One such target is the enzyme O-acetyltransferase A (OatA). This extracellular enzyme modifies the essential bacterial cell wall component peptidoglycan and thereby makes it resistant to the lytic action of lysozyme, our first line of defense against invading pathogens. It uses a catalytic triad of Ser-His-Asp to transfer acetyl groups specifically to the C-6 hydroxyl group of muramoyl residues within peptidoglycan. The overall structure of SpOatAC adopts an atypical α/β hydrolase fold, where the core parallel β-sheet contains five strands (β1 - β5) sandwiched between seven α-helices (α1–α7) forming a shallow and solvent exposed putative active site pocket.

Unequivocal identification of Ser438 in SpOatAC as the catalytic nucleophile was made using the mechanism-based, irreversible inhibitor of Ser esterases methanesulfonyl fluoride (MSF). SpOatAC treated with this reagent lacked detectable catalytic activity and X-ray crystallographic analysis of a native crystal soaked with MSF revealed the formation of a covalent adduct to Ser438 (described further below). To confirm the identification of the catalytic nucleophile and gain further insight into the enzyme’s mechanism of action, we determined the structure of MSF-inactivated SpOatAC (SpOatAC-MeS) at 2.1 Å resolution following modification of the native enzyme in cyrstallo with MSF. The MeS group is seen to form a covalent bond to the Oδ of Ser438 in a tetrahedral configuration and it is well defined in the electron density map. The overall structures of SpOatAC and SpOatAC-MeS are very similar (Cα RMSD: 0.327 Å over 178 residues), but several side chain displacements were observed in the active site on MeS binding. The most significant structural change involved the side chain of Asn491. The presence of the MeS adduct opens the active site, shifting the Nδ2 of Asn491 2 Å from its initial position away from Ser438 and displacing the water molecule w1. Other minor displacements occur in Ser438, Ser461, and His571 as a consequence of the steric effects imposed by the bound MeS. The methyl group of the MeS adduct appears to face the solvent adjacent to Val460, and the sulfonyl O2 (the structural mimic of an attacking water for hydrolytic activity; labeled O11 in the coordinate file) forms a weak H-bond (3.3 Å) to the imidazolium group of His571 while protruding into a hydrophobic pocket formed by Val490 and Val570.

> GIADGTMLIGDSVALRANTALQTALPGAQINAQVSVTTKTANEIMLNNSQNKFLPKTVVIATGVNNPENYKDDWDSIVKNLPKGHHMILVTPYEGDKTKETYAIVEKAAAYMRELAEKTPYITIADWNQVAKEHPEIWAGTDQVHFGSESSTIEAGAKLYADTIATALQTAQDKPVKSK> MAYFTGTANNPADLLAKVRVHAESLGWVTDRASASEWLCHNADGYWSFNAGANQFQMAGNTGFDNSLAWNAQPGNSVQNNPYSSKGPTVAQLSGGPFTRYHLFATAAYLHL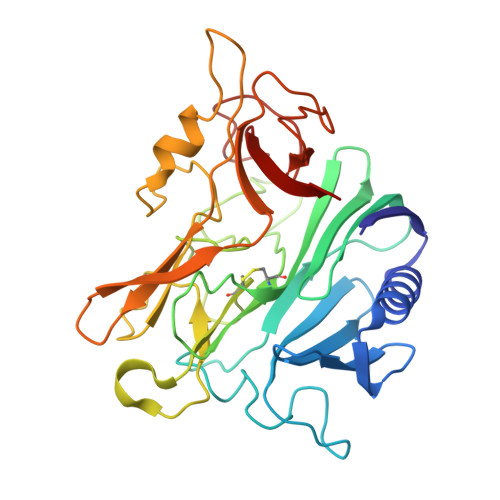HVEIAAGQFRPVMIGSLNKRGVGYTGGQYVCGSFIYTPGQALTNNWSSHPFDGYHIQYSNSSCMLRLDGLDGGPSPEWLPFDYTTNVPRRVVGPGRGNYSSQYHPDVGLIDASANELNSSTTTVPCAIYAFGAQQRSRYVGEVPDFGICNMAFLAPGDPLVVGSDTWRVYPLLQRGTATDFDSTSAWVGYCFRVVE>[4x]MAKDIGINSDPNSSSVDKLMKSSGVSNPTYTLVWKVWILAVTLYYAIRIPLTLVFPSLFSPLLPLDILASLALIADIPLDLAFESRRTSGRKPTLLAPSRLPDLLAALPLDLLVFALHLPSPLSLLSLVRLLKLISVQRSATRILSYRINPALLRLLSLVGFILLAAHGIACGWMSLQPPSENPAGTRYLSAFYWTITTLTTIGYGDITPSTPTQTVYTIVIELLGAAMYGLVIGNIASLVSKLDAAKLLHRERVERVTAFLSYKRISPELQRRIIEYFDYLWETRRGYEEREVLKELPHPLRLAVAMEIHGDVIEKVALFKGAGEEFIRDIILHLEPVIYGPGEYIIRAGEMGSDVYFINRGSVEVLSADEKTRYAILSEGQFFGEMALILRAPRTATVRARAFCDLYRLDKETFDRILSRYPEIAAQIQELAVRRKELESSGLVPRGSVKHHHH

SthK has functional similarity to eukaryotic cyclic nucleotide-modulated channels making it a bona fide model system to study specific mechanistic aspects of these channels. SthK also has the same architecture and similar sequence and structure as eukaryotic HCN and CNG channels, but unlike its eukaryotic counterparts, pure SthK protein can be easily produced in large enough quantities for structural and functional work. SthK has a voltage sensing domain, a pore domain, and a cytosolic cyclic nucleotide-binding domain (CNBD) that is connected to the pore via a helical C-linker. In all cyclic nucleotide-gated channels the connection between the C-linker and the CNBD is formed by a helix-loop-helix motif called the siphon. Interestingly, a proline is located at the end of the first siphon helix (Pro300 in SthK), which is conserved in HCN and SthK, but not CNG, channels.

Here, to overcome this heterogeneity and understand what the structure could look like with only one, defined configuration at Pro300, we solved the single-particle cryoEM structure of SthK P300A (all-trans Pro mimic) in lipid nanodiscs and in the presence of cAMP. In agreement with the low open probability of SthK P300A at 0 mV, we observed that the majority of SthK P300A particles (~90%), adopt a closed-state conformation (3.4 Å resolution), similar to cAMP-bound WT SthK13. Analysis of the major, closed conformation of SthK P300A, revealed that the siphon, where the mutation is located, has a slightly different conformation compared to WT SthK. However, the density in this area is weak, making a detailed comparison difficult. Interestingly though, the density in the siphon region of SthK P300A appears similar in resolution to the density around it, indicating less heterogeneity than in the WT channel, as one may expect if cis/trans Pro300 was contributing to the flexibility. Overall, the closed states of SthK P300A and WT SthK13 overlay with an RMSD of ~0.7 Å indicating that the structures are similar, but not identical. In this alignment, the cytosolic C-linker/CNBD domains in SthK P300A are now globally displaced by a small amount from the WT SthK structure (RMSD ~ 1.5 Å). This displacement is a rigid body movement, that brings the CNBDs in SthK P300A about 1–1.5 Å closer to the membrane compared to their position in WT SthK. The structure of SthK P300A in the closed state reveals a previously undetected conformation of SthK, which we hypothesize is what WT SthK with all-trans Pro300 would look like. Close inspection of the interface between adjacent CNBDs reveals subtle rearrangements in the closed-state of SthK P300A compared to WT SthK, raising the possibility that this energy could originate from different CNBD-CNBD interactions with cis or trans Pro300.Central to the purine metabolic pathway is inosine-5′-monophosphate dehydrogenase (IMPDH; EC 1.1.1.205), a rate-limiting enzyme catalyzing the NAD+-dependent oxidation of inosine-5′-monophosphate (IMP) to xanthosine 5′-monophosphate (XMP). Most of the IMPDHs share a conserved two-domain architecture consisting of a catalytic domain and a smaller regulatory cystathionine β-synthase (CBS) domain (also known as the Bateman module). The CBS domain serves as an allosteric regulatory module responding to the binding of nucleotide effectors. The enzyme is inhibited by both GTP and (p)ppGpp, which bind to the regulatory CBS domains and, via interactions with basic residues in hinge regions, lock the catalytic core domains in a compressed conformation.

The only extended MsmIMPDH structure was obtained from samples containing ATP in combination with the substrate IMP. The dataset of MsmIMPDH in the presence of ATP and IMP was highly heterogeneous, resulting in multiple 3D classes of MsmIMPDH octameric assemblies differing in their compression and extension range (Supplementary Fig. EM 6). Three distinct classes were refined: extended, compressed, and intermediate. The compressed structure closely resembled the compressed forms of apo and ATP-bound MsmIMPDH. The IMP molecule was only partially present, represented by weak densities observed for its phosphate and sugar moieties. In all our compressed structures, the Cys-loop, containing the catalytic Cys325 residue, adopted the inactive open conformation, but in the extended form, the active closed conformation prevailed, correlating with the presence of IMP.

>MSIAESSVPIAVPVPTGGDDPTKVAMLGLTFDDVLLLPAASDVVPATADTSSQLTKRIRLRVPLVSSAMDTVTESRMAIAMARAGGMGVLHRNLPVAEQAGQVETVKRSEAGMVTDPVTCSPDNTLAEVDAMCARFRISGLPVVDDTGELVGIITNRDMRFEVDQSKPVSEVMTKAPLITAKEGVSAEAALGLLRRHKIEKLPIVDGHGKLTGLITVKDFVKTEQFPLSTKDSDGRLLVGAAVGVGDDAWTRAMTLVDAGVDVLIVDTAHAHNRGVLDMVSRLKQAVGERVDVVGGNVATRAAAAALVEAGADAVKVGVGPGSICTTRVVAGVGAPQITAILEAVAACKPYGVPVIADGGLQYSGDIAKALAAGASTAMLGSLLAGTAESPGELIFVNGKQFKSYRGMGSLGAMQGRGAAKSYSKDRYFQDDVLSEDKLVPEGIEGRVPFRGPLGTVIHQLTGGLRAAMGYTGSATIEQLQQAQFVQITAAGLKESHPHDITMTVEAPNYYTR[8x]> METPEPRTTRTILVYMMANNSLNSFASKNIESMIEGATSKNLNGGNLIVYYAPAGSPPELLRIKEENGVVKKIHLKDYEKQNSADPDVMRSVIGEVVSQYPADSYGLVLWSHGTAWLPSDYQNKLK;> AFGQDGNNWMEIDDLAKGLPDDLFDFILFDACYMASVECTYELRNKAEYILASPTETMADGWPYEEMMPQLFATDLQLEKVGETFYNHYLNNTYPYATVSLTKTSELDNLKSAIHDILADKTESDIYSLDPKNMQRLEYLYRSPGMLYDFNDYIKQLATAEQYDRFISCLDKAVVY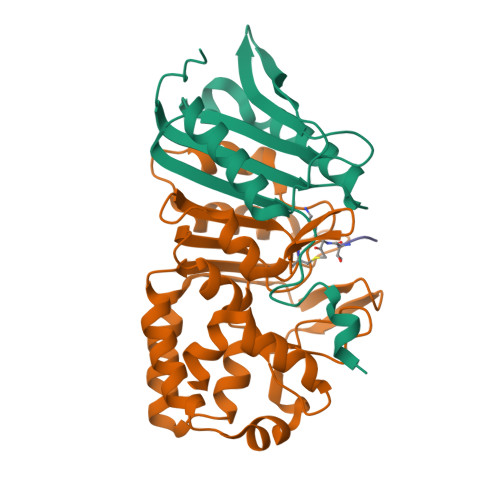KAHTPKSYYAAIGNALPIKSYCGLTIFVPQESLPKMLEWYKQRVGWYKAVYELEHHHHHH> GPG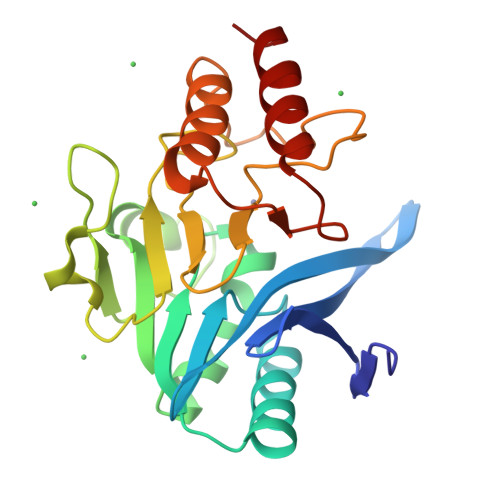DQRFGDLVFRQLAPNVWQHTSYLDMPGFGAVASNGLIVRDGGRVLVVDTAWTDDQTAQILNWIKQEINLPVALAVVTHAHQDKMGGMDALHAAGIATYANALSNQLAPQEGMVAAQHSLTFAANGWVEPATAPNFGPLKVFYPGPGHTSDNITVGIDGTDIAFGGCLIKDSKAKSLGNLGDADTEHYAASARAFGAAFPKASMIVMSHSAPDSRAAITHTARMADKLR>[2x]GPKGLVPGLVNLGNTCFMNSLLQGLSACPAFIRWLEEFTSQYSRDQKEPPSHQYLSLTLLHLLKALSCQEVTDDEVLDASCLLDVLRMYRWQISSFEEQDAHELFHVITSSLEDERDGSGSHWKSQHPFGVEFETTMKCTESEEEEVTKGKENQDSLSLSIPAATWGHPLTLDHCLHHFISQEEITKQSPTLQRNALYIKSSKISRLPQCLCIHLQRLSWSSHGTPLKRHEHVQFNEDLRLPLAGGRGQAYRLMAVVVHHGDMHSGHFVTYRRSPPSARNPLSTSNQWLWVSDDTVRKASLQEVLSSSAYLLFYERV

The mitochondrial deubiquitinase ubiquitin-specific protease (USP) 30 negatively regulates PINK1–parkin-driven mitophagy. Consequently, the mitochondrial deubiquitinase (DUB) ubiquitin-specific protease (USP)30 has emerged as a critical negative regulator of mitochondrial quality control due to its ability to remove ubiquitin from a subset of mitochondrial outer membrane proteins. By grafting structural elements of well-crystallizable human USP family members onto the periphery of the human USP30 protein, we generated stabilized and crystallizable protein constructs that retain DUB activity and the propensity to compound inhibition. In an iterative process, we explored 15 chimeric constructs starting with boundary design by structure superposition, design validation by AlphaFold2-based modeling, cloning, protein purification and biophysical characterization. This process is illustrated with four diverse chimeras: chimera 1 (USP30ch1) features the fingers of USP7, chimera 2 (USP30ch2) features the fingers of USP14, chimera 3 (USP30ch3) features the fingers of USP14 and the box 4–5 insertion of USP35, and chimera 4 (USP30ch4) features the fingers of CYLD.

The structure of USP30ch3 in complex with NK036 was solved to 2.75 Å following crystal optimization through fine screening and additive screening as well as data optimization through multicrystal averaging and anisotropic scaling. The asymmetric unit contained two copies of the protein–ligand complex. The ligand was surrounded only by USP30-encoded side chains as well as secondary structures generated by USP30 residues, with chimeric portions of the sequence spatially separated. NK036 was found to be engaged by both the palm and thumb subdomains and extensively surrounded by protein residues. The two central amide bonds of the ligand are contacted through a total of three hydrogen bonds by the protein: the backbone carbonyl group of Gln160 engages the anilinic NH proton, the carbonyl group of Met448 contacts the other amidic NH proton, and the carbonyl group of the fluorobenzoyl moiety engages the Ala162 nitrogen. These polar interactions give rise to a star-like tripartite geometry of NK036 with the hydrophobic portions of the ligand extending into three separate areas:The fluorobenzoyl ring binds into a hydrophobic pocket formed by Leu328, Tyr495 and Phe453 as well as aliphatic portions of the Arg327 and Lys338 side chains. While the catalytic residues of USP30 are not contacted by the inhibitor, we observed that the catalytic triad was not aligned in the inhibitor-bound state, as the catalytic histidine was flipped out. The superposition also revealed large and surprising conformational changes of the switching loop that allow the N-tert-butyl-benzenesulfonamide group to bind deeply within the thumb subdomain. Notably, Phe157 moves more than 18 Å and takes the place of Trp152, which is pushed out toward the fingers.6-[(5-fluoropyridin-2-yl)amino]-N-methyl-4-{[2-(methylsulfonyl)phenyl]amino}pyridine-3-carboxamide | C19 H18 F N5 O3 S | 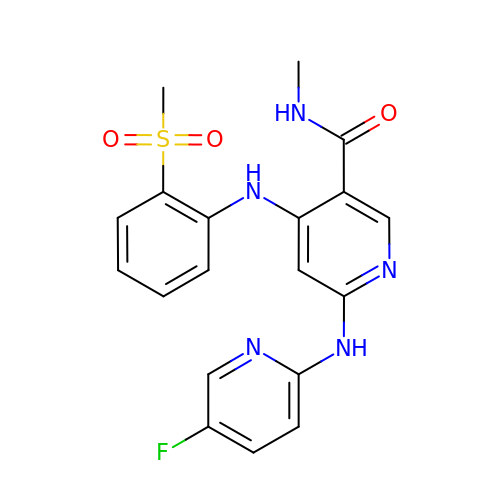SYYQNYIBIFOCPS-UHFFFAOYSA-N> AKCVSYGVAQIKAPALHSQGYTGSNVKVAVLASGIDSSHPDLNVAGGASFVPSETNPFQDNNSHGTHVAGTVLAVAPSASLYAVKVLGADGSGQASWIINGIEWAIANNMDVINMSLGSPSGSAALKAAVDKAVASGVVVVAAAGNSGTSGSSS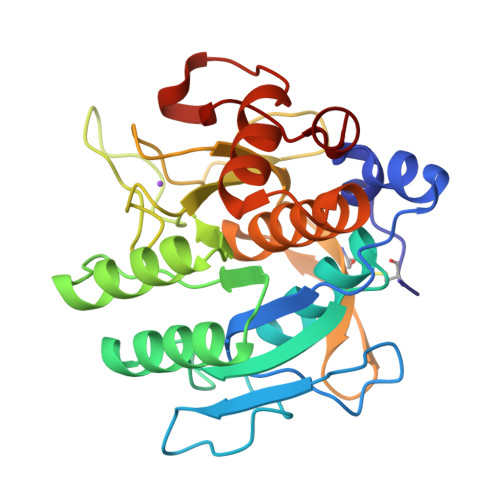TVSYPAKYPSVIAVGAVDSSNQRAPFSSVGPELDVMAPGVSICSTLPGGKYGALSGTSMASPHVAGAAALILSKHPNWTNTQVRSSLENTATKLGDSFYYGKGLINVEAAAQ> SNAEIKIGITMSASGPGAALGQPQSKTVAALPKEIGGEKVTYFALDDESDPTKAAQNARKLLSEEKVDVLIGSSLTPVSLPLIDIAAEAKTPLMTMAAAAILVAPMDERRKWVYKVVPNDDIMAEAIGKYIAKTGAKKVGYIGFSDAYGEGYYKVLAAAAPKLGFELTTHEVYARSDASVTGQVLKIIATKPDAVFIASAGTPAVLPQKALRERGFKGAIYQTHGVATEEFIKLGGKDVEGAIFAGEAFSGAEDMPADSPFRKVKARFVDAYKAANGGAAPTIFGVHLWDSMTLVENAIPAALKAAKPGTPEFRAAIR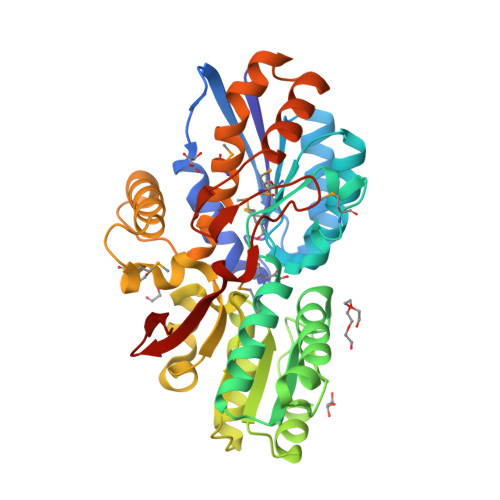DQIEKSKDLALNNGLSNMTPDNHNGYDERSAFLIEIRDGAFRLKQ>[2x]SVKLAGNSSLCPVSGWAIYSKDNSVRIGSKGDVFVIREPFISCSPLECRTFFLTQGALLNDKHSNGTIKDRSPYRTLMSCPIGEVPSPYNSRFESVAWSASACHDGINWLTIGISGPDNGAVAVLKYNGIITDTIKSWRNNILRTQESECACVNGSCFTVMTDGPSNGQASYKIFRIEKGKIVKSVEMNAPNYHYEECSCYPDSSEITCVCRDNWHGSNRPWVSFNQNLEYQIGYICSGIFGDNPRPNDKTGSCGPVSSNGANGVKGFSFKYGNGVWIGRTKSISSRNGFEMIWDPNGWTGTDNNFSIKQDIVGINEWSGYSGSFVQHPELTGLDCIRPCFWVELIRGRPKENTIWTSGSSISFCGVNSDTVGWSWPDGAELPFTIDK

NA, which is a sialidase, catalyzes hydrolysis of terminally linked sialic acid and functions as the receptor-destroying element of influenza A and B viruses. Additionally, influenza A NA is further classified into two groups: group 1 (N1, N4, N5 and N8) and group 2 (N2, N3, N6, N7 and N9), based upon primary sequence. Group 1 NAs contain a 150-cavity (formed by amino acids 147–151 of the 150-loop) in their active site, whereas group 2 NAs lack this cavity. NA inhibition assays were carried out and complex crystal structures were solved for laninamivir, laninamivir octanoate, zanamivir and oseltamivir in order to elucidate the structural basis of their inhibition.

Laninamivir octanoate complex structures with p09N1 and p57N2 were solved at 1.6 Å and 2.2 Å, respectively, demonstrating that the laninamivir octanoate prodrug can also directly inhibit NA without further processing. Surprisingly, the p09N1-laninamivir octanoate complex shows a completely different binding mode: p09N1 adopts a Glu276-Arg224 salt bridge in its laninamivir octanoate complex, forming a hydrophobic pocket that is also necessary to accommodate oseltamivir. The rotation of p09N1 Glu276 places it out of range for hydrogen bonding with the 8-OH and 9-ester-O of laninamivir octanoate. Instead, the p09N1-laninamivir octanoate 9-ester-O forms a unique hydrogen bond with Asn294. Additionally, 09N1 Ser247 forms another hydrogen bond with the laninamivir octanoate 9-ester-O at 3.4–3.5 Å. Still, the Glu276 rotation results in less hydrogen bonding in the p09N1-laninamivir octanoate complex compared to p57N2. Furthermore, in p09N1, the position 7-methoxy of laninamivir octanoate is also oriented slightly away from its N-acetyl group relative to laninamivir and there is additional electron density pointing toward the ring, indicating lower stability of the p09N1-laninamivir octanoate complex. In all of our NA complex structures, bond distances in each molecule of the asymmetric units are very similar, however in the p09N1-laninamivir octanoate structure some greater differences are observed between molecule A and B in the asymmetric unit, which further reflects the lower stability of the prodrug's octanoyl ester in p09N1. In p09N1 molecule A, the distance between the 9-ester-O and Asn294 is 2.64 Å, however in molecule B the distance is much further at 3.93 Å. In a similar manner, the group 1 Tyr252 side chain promotes the native His274 to occupy a position where it can participate in a hydrogen bond network with Glu276 and Arg224 as observed in our 09N1-laninamivir octanoate structure.>MGTPALDRAKLLKQYRKARKRLFMFDYDGTLTPIVKDPQAAIPSDRVLRTLKTLAADPRNA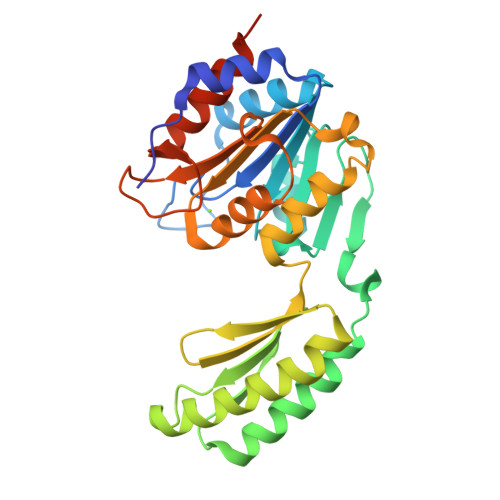VWIISGRDQAFLDEWMGHIPELGLSAEHGCFIRQPRSDDWENLAESSDMGWQKEVMEVFQHFTERTQGSFIERKRVALTWHYRRADPEYGAFQARECRKMLEETVAKRWEVEVMAGKANLEVRPTFVNKGFIAARLVQEYGTDPAQAPEFVLCLGDDFTDEDMFRALKKSGLPAGHVFSVTVGASSKQTEASWHLLEPADVIGTISMLNNSSSAQEYLEHHHHHH[2x]> SRPLSDQEKRKQISVRGLAGVENVTELKKNFNRHLHFTLVKDRNVATPRDYYFALAHTVRDHLVGRWIRTQQHYYEKDPKRIYYLSLEFYMGRTLQNTMVNLALENACDEATYQLGLDMEELEEIEEDAGLGNGGLGRLAACFLDSMATLGLAAYGYGIRYEFGIFNQKICGGWQMEEADDWLRYGNPWEKARPEFTLPVHFYGRVEHTSQGAKWVDTQVVLAMPYDTPVPGYRNNVVNTMRLWSAKAPNDFNLKDFNVGGYIQAVLDRNLAENISRVLYPNDNFFEGKELRLKQEYFVVAATLQDIIRRFKSSKFGCRDPVRTNFDAFPDKVAIQLNDTHPSLAIPELMRVLVDLERLDWDKAWEVTVKTCAYTNHTVLPEALERWPVHLLETLLPRHLQIIYEINQRFLNRVAAAFPGDVDRLRRMSLVEEGAVKRINMAHLCIAGSHAVNGVARIHSEILKKTIFKDFYELEPHKFQNKTNGITPRRWLVLCNPGLAEIIAERIGEEYISDLDQLRKLLSYVDDEAFIRDVAKVKQENKLKFAAYLEREYKVHINPNSLFDVQVKRIHEYKRQLLNCLHVITLYNRIKKEPNKFVVPRTVMIGGKAAPGYHMAKMIIKLITAIGDVVNHDPVVGDRLRVIFLENYRVSLAEKVIPAADLSEQISTAGTEASGTGNMKFMLNGALTIGTMDGANVEMAEEAGEENFFIFGMRVEDVDRLDQRGYNAQEYYDRIPELRQIIEQLSSGFFSPKQPDLFKDIVNMLMHHDRFKVFADYEEYVKCQERVSALYKNPRE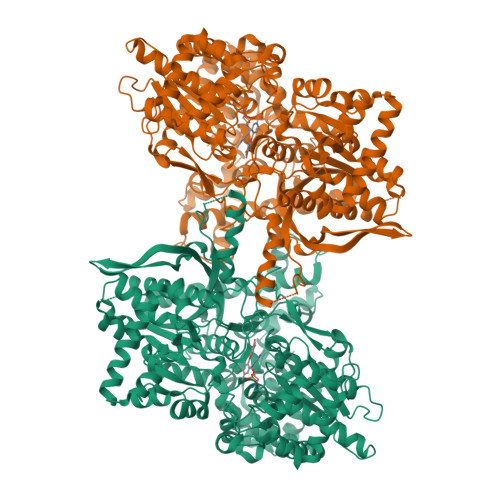WTRMVIRNIATSGKFSSDRTIAQYAREIWGVEPSRQRLPAPDEKIP> HLEVVKLLLEAGADVNAQ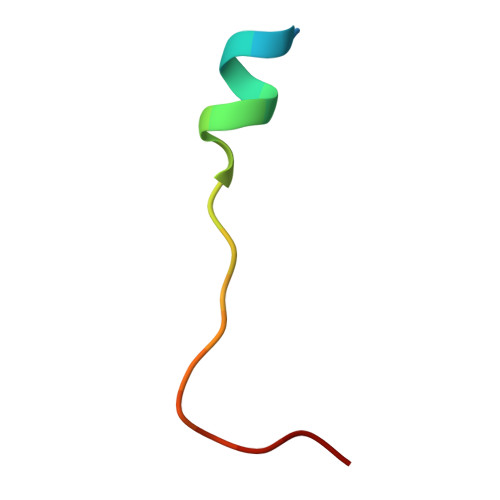DK> MEYGVLSVILVIVVAFLAGLEGILDQWQFHQPIIACSLIGIVTGHAS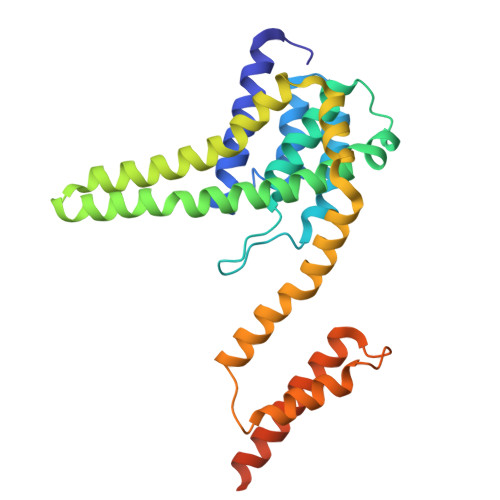AGIILGGSLQLIALGWANVGAAVAPDAALASIASSILMVQSNNFDLTHIMGTIVPAAILLATAGLVLTTLVRMLSVVLVHQADRAAENGSYSGVEMWHFIALICQGLRIAIPAGLLLVISPDAIQKALAAIPPVISGGLAVGGGMVVAVGYAMVINLMATREVWPFFFLGFALAPISELTLIATGVLGVVIAIVYLNLQASGGSGNGTASSSGDPIGDILNDY> HHHHHHMGRTVVVLGGGISGLAASYHLSRAPCPPKVVLVESSERLGGWIRSVRGPNGAIFELGPGGIRPAGALGARTLLLVSELGLDSEVLPVRGDHPAAQNRFLYVGGALHALPTGLRGLLRPSPPFSKPLFWAGLRELTKPRGKEPDETVHSFAQRRLGPEVASLAMDSLCRGVFAGNSRELSIRSCFPSLFQAEQTHRSILLGLLLGAGRTPQPDSALIRQALAERWSQWSLRGGLEMLPQALETHLTSRGVSVLRGQPVCGLSLQAEGRWKVSLRDSSLEADHVISAIPASVLSELLPAEAAPLARALSAITAVSVAVVNLQYQGAHLPVQGFGHLVPSSEDPGVLGIVYDSVAFPEQDGSPPGLRVTVMLGGSWLQTLEASGCVLSQELFQQRAQEAAATQLGLKEMPSHCLVHLHKNCIPQYTLGHWQKLESARQFLTAHRLPLTLAGASYEGVAV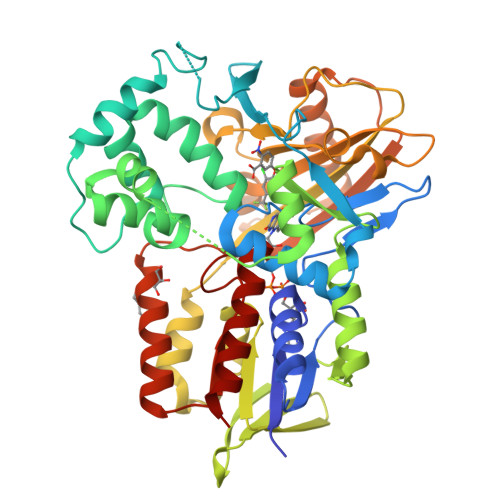NDCIESGRQAAVSVLGTEPNS>[8x]MNNNDIEYNAPSEIKYIDVVNTYDLEEEASKVVPHGGFNYIAGASGDEWTKRANDRAWKHKLLYPRLAQDVEAPDTSTEILGHKIKAPFIMAPIAAHGLAHATKEAGTARAVSEFGTIMSISAYSGATFEEISEGLNGGPR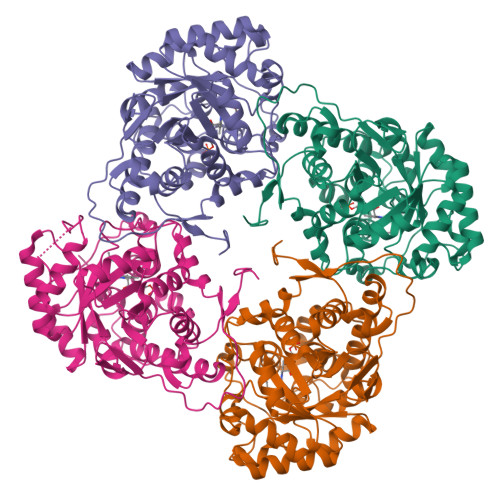WFQIYMAKDDQQNRDILDEAKGDGATAIILTADSTVSGNRDRDVKNKFVYPFGMPIVQRYLRGTAEGMSLNNIFGASKQKISPRDIEEIAAHSGLPVFVKGIQHPEDADMAIKAGASGIWVSNHGARQLYEAPGSFDTLPAIAERVNKRVPIVFDSGVRRGEHVAKALASGADVVALGRPVLFGLALGGWQGAYSVLDYFQKDLTRVMQLTGSQNVEDLKGLDLFDNPYGYEY>[6x]MILAAKKKAVAVLKGNSAVEGVVTLTQEEDGPTTVNVRITGLTPGPHGF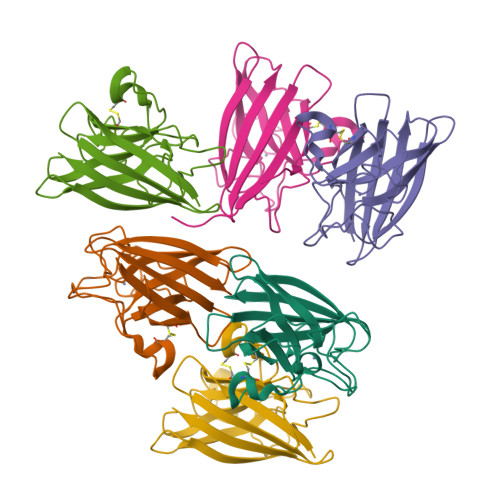HLHEFGDTTNGCISTGPHFNPKGLTHGAPEDEIRHAGDLGNIVANADGVAEVTIVDNQIPLTGPNAVVGRAFVVHELEDDLGKGGHELSLSTGNAGGRLACGVIGLTPT> G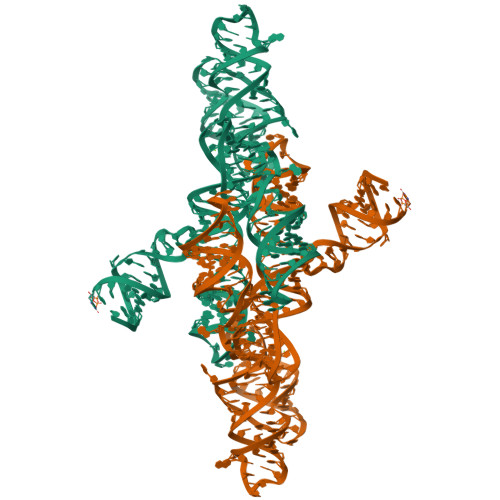GCGCUGUGUCGCAAUCUGCGAAGGGCGUCGUCGGCCCGAGCGGUAGUAAGCAGGGAACUCACCUCCAAUGAAACACAUUGUCGUAGCAGUUGACUACUGUUAUGUGAUUGGUAGAGGCUAAGUGACGGUAUUGGCGUAAGCCAAUACCGCGGCACAGCACAAGCCCGCUUGCGAGAUUACAGCGC> PTRNESINPWVLTGFADAEGSFILRIRNNNKSSAGYSTELGFQITLHKKDKSILENIQSTWKVGVIANSGDNAVSLKVTRFEDLRVVLNHFEKYPL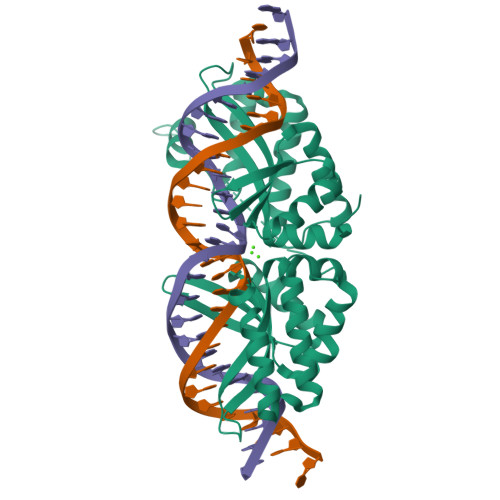ITQKLGDYLLFKQAFSVMENKEHLKIEGIKRLVGIKANLNWGLTDELKEAFVASGGENIFVASGGERSLINKNIPNSGWLAGFTSGEGCFFVSLIKSKSKLGVQVQLVFSITQHARDRELMDNLVTYLGCGYIKEKKKSEFSWLEFVVTKFSDIKDKIIPVFQENNIIGVKLEDFEDWCKVAKLIEEKKHLTESGLEEIRNIKLNMNKGRVL>[4x]MSEVVSFSFTKFNPNPKDIILQGDALVTSKGKLQLTKVKDGKPVDHSLGRALYAAPIHIWDDSTDRVASFATSFSFVVEAPD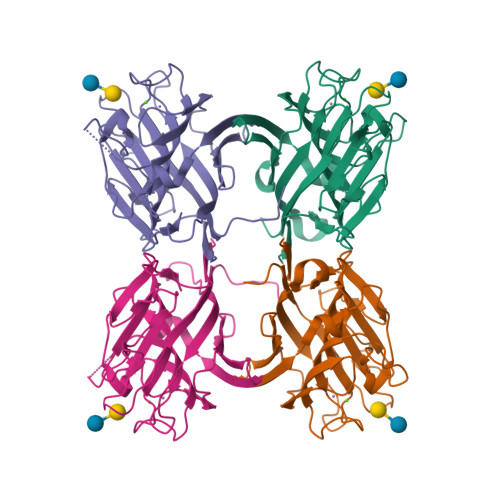ESKTADGIAFFLAPPDTQPQKDGGFLGLFNDSNKSIQTVAVEFDTFSNTWDPSARHIGINVNSIESMKYVKWGWENGKVANVYISYEASTKTLTASLTYPSNATSYIVSANVDLKSALPEWVRVGFSATSGLSRDHVETHDVLDWSFTSTLQAPSDDSN>GPHMSDHKFLTQ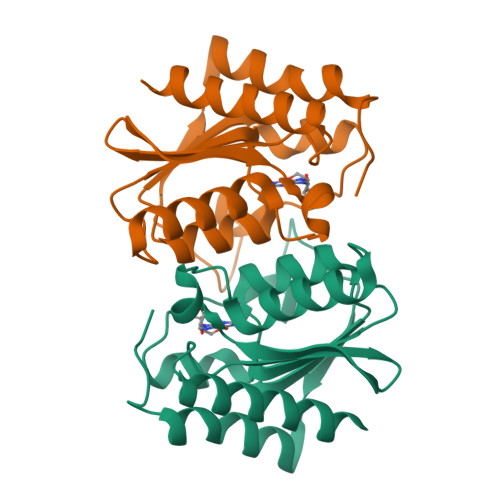AVEEAYKGVDCGDGGPFGAVIVHNNEVVASCHNMVLKYTDPTAHAEVTAIREACKKLNKIELSECEIYASCEPCPMCFGAIHLSRLKRLVYGAKAEAAIAIGFDDFIADALRGTGVYQKSSLEIKKADGNGAAIAEQVFQNTKEKFRLY[2x]>MKKYVCTVCGYEYDPAEGDPDNGVKPGTAFEDVPADWVCP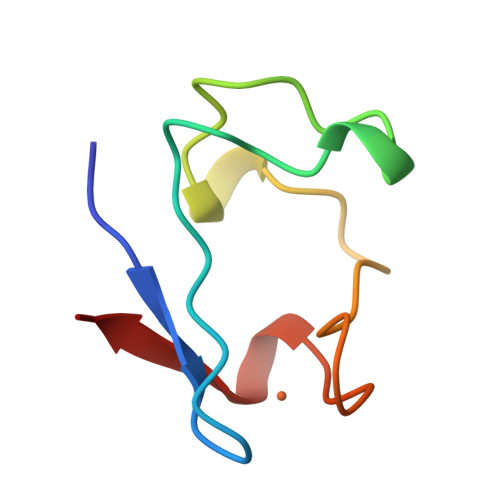ICGAPKSEFEPA[3x]>GDTKEQRILRYVQQNAKPGDPQSVLEAIDTYCTQKEWAMNVGDAKGQIMDAVIREYSPSLVLELGAYCGYSAVRMARLLQPGARLLTMEINPDCAAITQQMLNFAGLQDKVTILNGASQDLIPQLKKKYDVDTLDMVFLDHWKDRYLPDTLLLEECGLLRKGTVLLADNVIVPGTPDFLAYVRGSSSFECTHYSSYLEYMKVVDGLEKAI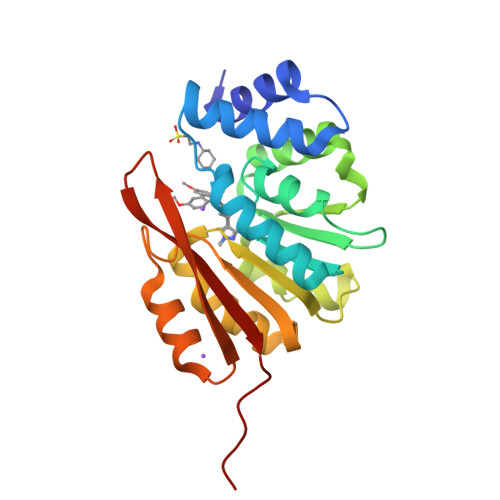YQGPSSPDKS[2x]> AA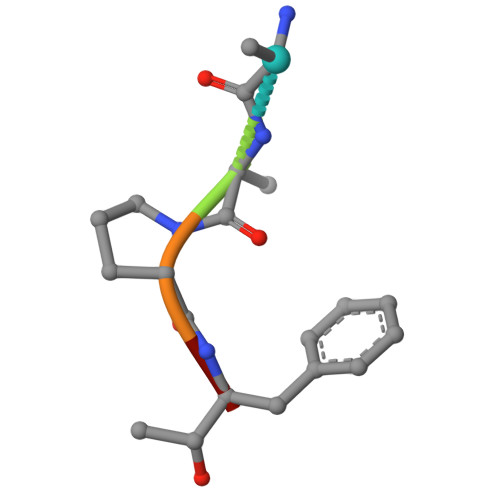PFX>ASVDTMNARNTQFTKAFHALKQNAGSHSPSMEDLKKMFPTLEIKIDACYLSNPYASELVLDYIDRELIQTNAYKKVLTHYPSQQRSLQKVMAESLHVKPENIFIGNGATEIIQMLLQQEEVQKVALMIPTFSSYYEFVGKGCEVVYFPLNERDDYSFDADKYCQFIENEQPDTVVLINPNNPNGAYLSLEKMHILLKRLAFVPRIIIDESFIHFAYEDEALTCLSSTVLFDMYPNVIIVKSLSKDFGIAGVRLGYALMDSRKIDALLEHGFLWNINGIGEYCLRLFVREDFLKRYEEARKQYIKEMCRFKEALLGIENVYVYPSMAN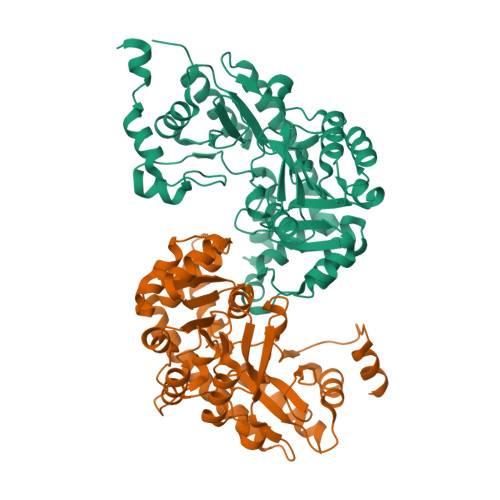FVMLKLPSRIKASFVISALLVEYGIYVRTMADKIGVEGECIRIAGRTREENNCIVMALKSILKDSK[2x]>GPLDVIRCICGLYKDEGLMIQCDKCMVWQHCDCMGVNSDVEHYLCEQCDPRPVDRE[2x];>ARTKQTARKST[2x]

The histone H3K36-specific methyltransferase ASH1L plays a critical role in development and is frequently dysregulated in human diseases, particularly cancer. ASH1L itself functions as a specific methyltransferase: it methylates lysine 36 of histone H3 producing mono- and di-methylated epigenetic marks H3K36me1/214,15. There is no information available about the N-terminal 2,000 amino acids of ASH1L, though several domains have been identified in the C-terminal part, which contains the catalytic SET (Su(var), E(z), Trithorax) domain, followed by a bromodomain (BD), a plant homeodomain (PHD) finger and a bromo-adjacent homology (BAH) domain. We find that ASH1LPHD recognizes H3K4me2/3, whereas the neighboring ASH1LBD and ASH1LBAH have DNA binding activities.

Titration of H3K4me3 or H3K4me2 peptide (residues 1-12 of H3) into the ASH1LPHD NMR sampl led to large chemical shift perturbations (CSPs) in 1H,15N heteronuclear single quantum coherence (HSQC) spectra of ASH1LPHD. These changes were in the intermediate exchange regime on the NMR time scale, indicating tight binding. In agreement, a 1-2 μM binding affinity of ASH1LPHD to di- and trimethylated peptides was measured by tryptophan fluorescence and MST. We note that this affinity is in the range of binding affinities exhibited by the majority of histone binding modules, suggesting that the recognition of H3K4me2/3 by ASH1LPHD is physiologically relevant. In contrast, the association of ASH1LPHD with H3K4me1 or H3K4me0 peptides was weaker (Kds of 119 μM and 1900 μM, respectively). To gain insight into the molecular mechanism of the recognition of H3K4me3/2, we co-crystallized ASH1LPHD with H3K4me3 and H3K4me2 peptides and determined a 1.3 Å resolution crystal structure of the ASH1LPHD:H3K4me3 complex and a 1.9 Å resolution crystal structure of the ASH1LPHD:H3K4me2 complex. The ASH1LPHD fold is stabilized by two zinc-binding clusters and a twisted double-stranded anti-parallel β-sheet. The structure of the ASH1LPHD-H3K4me3 complex overlays well with the structure of the ASH1LPHD-H3K4me2 complex (rmsd of 0.1 Å), as well as with the structure of the ING2PHD-H3K4me3 complex (rmsd of 1 Å), pointing to a conserved mode of the methyllysine recognition. Like in the ASH1LPHD:H3K4me2 complex, in the ASH1LBD-PHD:H3K4me2 complex, the peptide forms a third antiparallel β strand to the existing β-sheet of ASH1LPHD. Overall, the two structures superimpose well (rmsd of 0.9 Å), indicating that no major conformational change occurs in ASH1LPHD when it is linked to ASH1LBD.> GAGCAACUUAGGAUUUUAGGCUCCCCGGCGUGUCUCGAACCAUGCCGGGCCAAACCCAUAGGGCUGGCGGUCCCUGU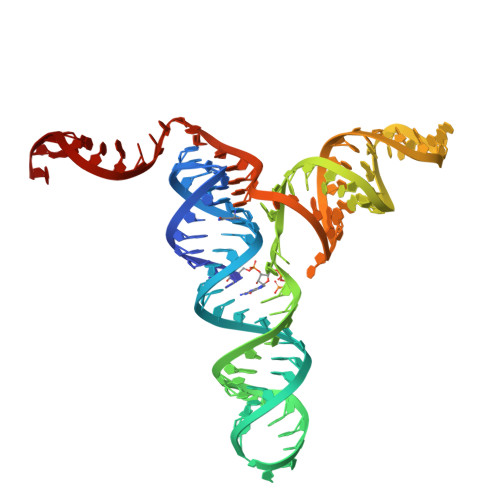GCGGUCAAAUUCAUCCGCCGGAG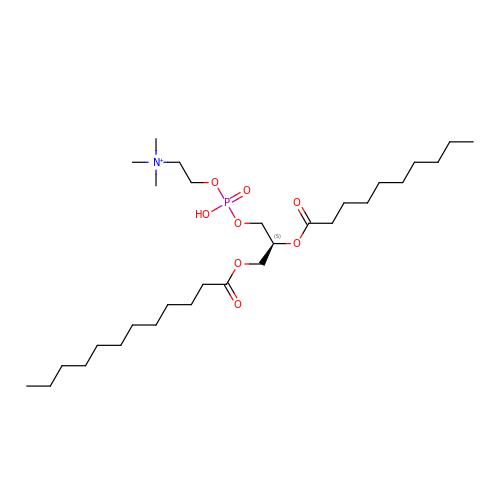2-[[(2~{S})-2-decanoyloxy-3-dodecanoyloxy-propoxy]-oxidanyl-phosphoryl]oxyethyl-trimethyl-azanium | C30 H61 N O8 P | YCHNJZJVKCSKTN-NDEPHWFRSA-O> GSAMGMSNTQAERSIIGMIDMFHKYTRRDGKIDKPSLLTMMKENFPNFLSACDKKGTNYLADVFEKKDKNEDKKIDFSEFLSLLGDIATDYHKQSHGAAPCSGGSQAAA

S100 proteins are a family of small, EF-hand containing calcium-binding signaling proteins that are implicated in many cancers. Hallmarks of the S100 protein family include their small size (~ 100 aa) and the presence of a canonical (calmodulin-like) EF-hand motif and a non-canonical (S100-specific) EF-hand motif. While most S100 proteins share moderate sequence identity, S100A7 and S100A15 are 93% identical in sequence yet intriguingly display divergent functions. Intriguingly, however, S100A7 and S100A15 serve distinct roles in inflammatory skin disease; S100A7 signals through the receptor for advanced glycation products (RAGE) in a zinc-dependent manner, while S100A15 signals through a yet unidentified G-protein coupled receptor in a zinc-independent manner.

To confirm that the substitution of Asp24 with a glycine was solely responsible for the unique zinc-binding site observed in S100A15, we generated the D24G variant of S100A7. S100A7D24G eluted as a dimer from the SEC, and crystallized with one monomer in the asymmetric unit of the tetragonal cell. Diffraction data was collected to a resolution of 1.6 Å and the structure solved by molecular replacement. The S100A7D24G and S100A15 structures aligned closely with an r.m.s.d of 0.719 Å over 96 Cα atoms. Subtle adjustments were observed in the orientation of the histidine ligands, due to differential packing of surface loops between the monoclinic and tetragonal crystal forms. To validate the modeling of zinc at the dimer interface, we calculated an anomalous difference map using data collected at the zinc edge of 1.2482 nm. A large anomalous difference peak (>12 σ) was observed where the zinc had been modeled confirming the identity of the bound metal as zinc. While crystallization of S100A15 was completed in the presence of zinc, S100A7D24G was crystallized in the absence of zinc, and yet zinc binding was observed in the same geometry. These observations indicate that the zinc-binding observed in the S100A15 is not an artifact. Similar to S100A15, a chloride ion was modeled as the exogenous fourth ligand to complete the distorted tetrahedral geometry.> MTKTTDDNIIVGLDIGTATVSALVGEVLPDGQVNIIGAGSSPSRGMDKGGVNDLESVVKSVQRAVDQAELMAECQISSVFISLSGKHIASRIEKGMGTISEEEVSQDDMDRAIHTAKSIKIGDEQRILHVIPQEFTIDYQEGIKNPLGLSGVRMEVSVHLISCHNDMARNIIKAVERCGLKVEQLVFSGLASSNAVITEDERELGVCVVDIGAGTMDISIWTGGALRHTEVFSYAGN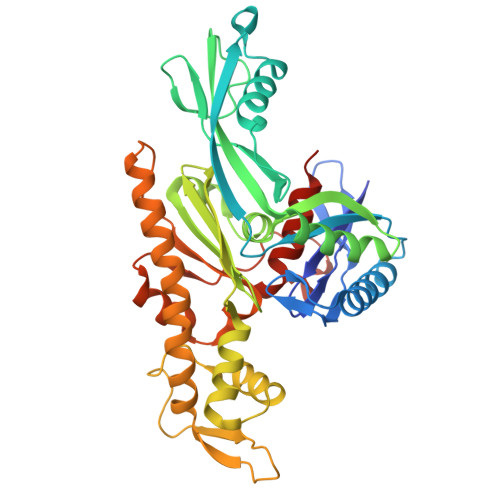AVTSDIAFAFGTPLSDAEEIKVKYGCALSELVSKDDTVNVPSVGGRPSRSLQRQTLAEVIEPRYTELMGLVNQTIDNVQAKLRENGVKHHLAAGVVLTGGAAQIEGVVECAERVFRNQVRVGKPLEVSGLTDYVKEPYHSTAVGLLHYARDSQDNDDND>GSHMNGNVALSDGHNTAEEDMEDDTSWRSEATFQFTVERFSRLSESVLSPPCFVRNLPWKIMVMPRFYPDRPHQKSVGFFLQCNAESDSTSWSCHAQAVLKIINYRDDEKSFSRRISHLFFHKENDWGFSNFMAWSEVTDPEKGFIDDDKVTFEVFVQADAPHGVAWDSKKHTGYVGLKNQGATCYMNSLLQTLFFTNQLRKAVYMMPTEGDDSSKSVPLALQRVFYELQHSDKPVGTKKLTKSFGWETLDSFMQHDVQELCRVLLDNVENKMKGTCVEGTIPKLFRGKMVSYIQCKEVDYRSDRREDYYDIQLSIKGKKNIFESFVDYVAVEQLDGDNKYDAGEHGLQEAEKGVKFLTLPPVLHLQLMRFMY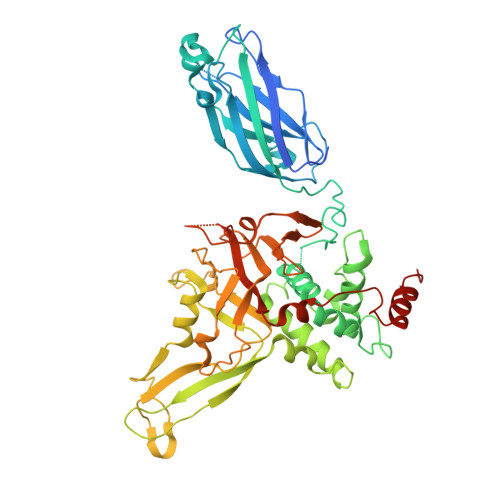DPQTDQNIKINDRFEFPEQLPLDEFLQKTDPKDPANYILHAVLVHSGDNHGGHYVVYLNPKGDGKWCKFDDDVVSRCTKEEAIEHNYGGHDDDLSVRHCTNAYMLVYIRESKLSEVLQAVTDHDIPQQLVERLQEEKRIEAQKRKERQE[2x]>GSVPDEWEVAREKITMSRELGQGSFGMVYEGVAKGVVKDEPETRVAIKTVNEAASMRERIEFLNEASVMKEFNCHHVVRLLGVVSQGQPTLVIMELMTRGDLKSYLRSLRPEMENNPVLAPPSLSKMIQMAGEIADGMAYLNANKFVHRDLAARNCMVAEDFTVKIGDFGMTRDIYETDYYRKGGKGLLPVRWMSPESLKDGVFTTYSDVWSFGVVLWEIATLAEQPYQGLSNEQVLRFVMEGGLLDKPDNCPDMLFELMRMCWQYNPKMRPSFLEIISSI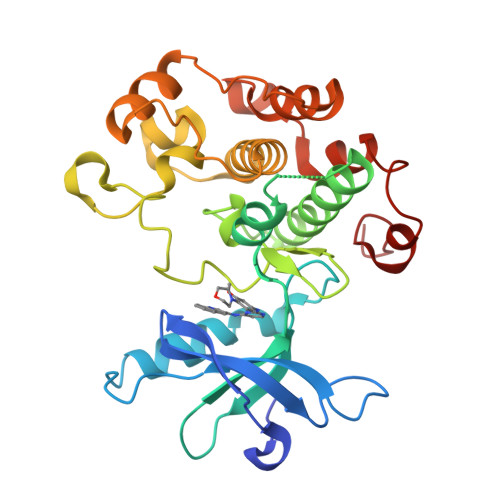KEEMEPGFREVSFYYSEENK[4x]>[4x]GSVIDPSELTFVQEIGSGQFGLVHLGYWLNKDKVAIKTIREGAMSEE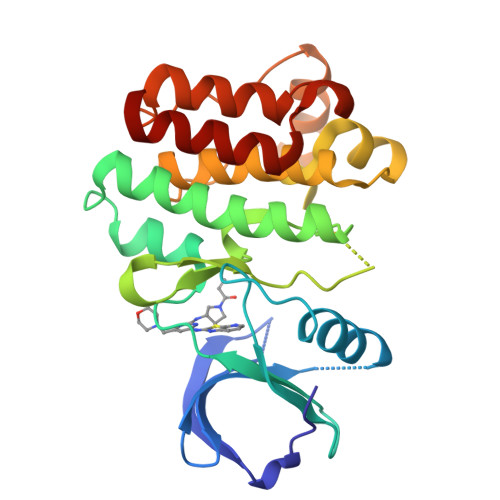DFIEEAEVMMKLSHPKLVQLYGVCLEQAPICLVFEFMEHGCLSDYLRTQRGLFAAETLLGMCLDVCEGMAYLEEACVIHRDLAARNCLVGENQVIKVSDFGMTRFVLDDQETSSTGTKFPVKWASPEVFSFSRYSSKSDVWSFGVLMWEVFSEGKIPYENRSNSEVVEDISTGFRLYKPRLASTHVYQIMNHCWKERPEDRPAFSRLLRQLAEIAESGL> SPQPLEQIKLSESQLSGRVGMIEMDLASGRTLTAWRADERFPMMSTFKVVLCGAVLARVDAGDEQLERKIHYRQQDLVDYSPVSEKHLADGMTVGELCAAAITMSDNSAANLLLATVGGPAGLTAFLRQIGDNVTR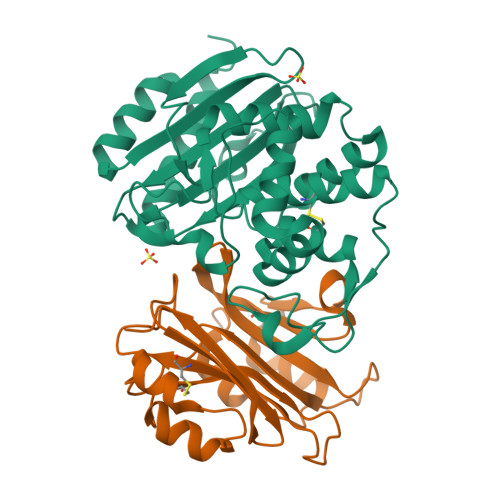LDRWETELNEALPGDARDTTTPASMAATLRKLLTSQRLSARSQRQLLQWMVDDRVAGPLIRSVLPAGWFIADKTGAGERGARGIVALLGPNNKAERIVVIYLRDTPASMAERNQQIAGIGAALIEHWQR;> AGVMTGAKFTQIQFGMTRQQVLDIAGAENCETGGSFGDSIHCRGHAAGDYYAYATFGFTSAAADAKVDSKSQMKLLAPSAPTLTLAKFNQVTVGMTRAQVLATVGQGSCTTWSEYYPAYPSTAGVTLSLKCFDVDGYSSTGFYRGMAHLWFTDGVLQGKRQWDLV>MSLRIGVIGLGRIGTIHAENLKMIDDAILYAISDVREDRLREMKEKLGVEKAYKDPHELIEDPNVDAVLVCSSTNTHSELVIACAKAKKHVFCEKPLSLNLADVDRMIEETKKADVILFTGFNRRFDRNFKKLKEAVENGTIGKPHVLRITSRDPAPPPLDYIRVSGGIFLDMTIHDFDMARYIMGEEVEEVFADGSVLVDEEIGKAGDVDTAVVVLRFKSGALGVIDNSRRAVYGYDQRIEVFGSKGRIFADNVRETTVVLTDEQGDRGSRYLY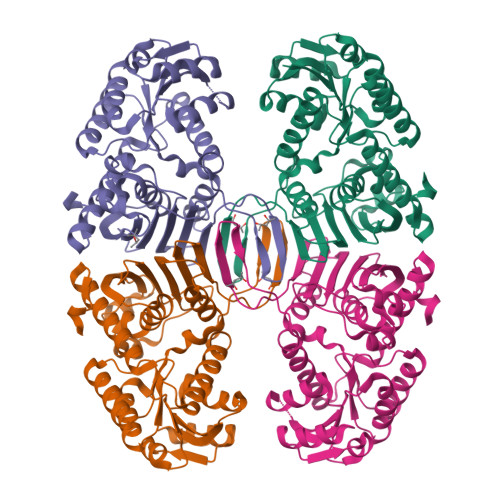FFLERYRDSYLEELKTFIKNVKSGEPPAVSGEDGKMALLLGYAAKKSLEEKRSVKLEEVIGEGHHHHHH[4x]1-cyanocyclohexyl (3S,5'R)-2-oxo-1,2-dihydrospiro[indole-3,3'-pyrrolidine]-5'-carboxylate | C19 H21 N3 O3 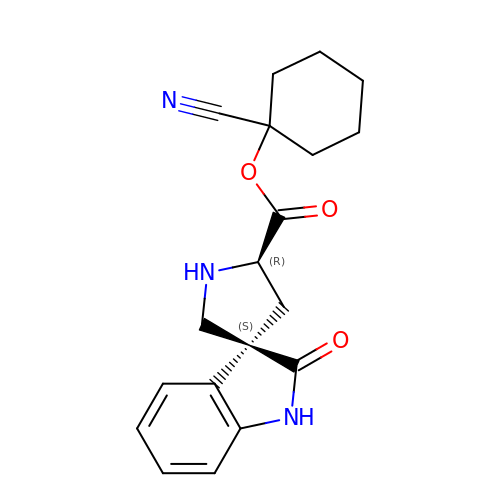| VRCMTLQTPNLTIN-DNVCBOLYSA-N> NLQPLETTITDVERFKDTVTLELSCPSCDKRFPFGGIVSSNYYRVSYNGLQCKHCEQLFTPLQLTSQIEHSIRAHISLYYAGWLQCDDSTCGIVTRQVSVFGKRCLNDGCTGVMRYKYSDKQLYNQLLYFDSLFD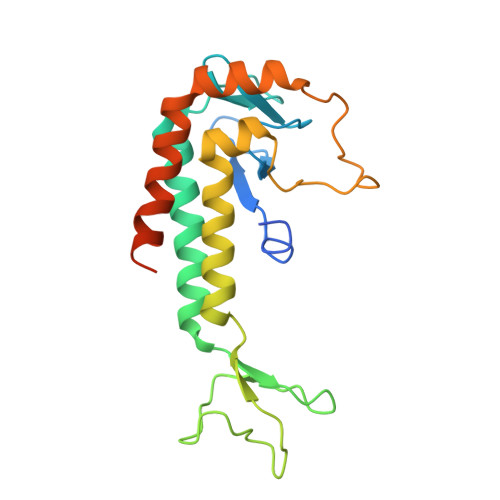CEKNKKQELKPIYLPDDLDYPKEQLTESSIKALTEQNRELMETGRSVVQKYLNDCGRRYVDMTSIFDFMLN>MKLQLVAVGTKMPDWVQTGFTEYLRRFPKDMPFELIEIPAGKRGKNADIKRILDKEGEQMLAAAGKNRIVTLDIPGKPWDTPQLAAELERWKLDGRDVSLLIGGPEGLSPACKAAAEQSWSLSALTLPHPLVRVLVAE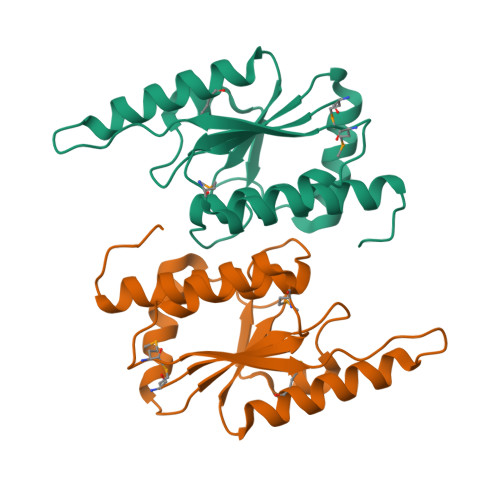SLYRAWSITTNHPYHRE[2x]> MFEARLVQGSILKKVLEALKDLINEACWDISSSGVNLQSMDSSHVSLVQLTLRSEGFDTYRCDRNLAMGVNLTSMSKILKCAGNEDIITLRAEDNADTLALVFEAPNQEKVSDYEMKLMDLDVEQLGIPEQEYSCVVKMPSGEFARICRDLSHIGDAVVISCAKDGVKFSASGELGNGNIKLSQTSNVDKEEEAVTIEMNEPVQLTFALRYLNFFTKATPLSSTVTLSMSADVPLVVEYKIADMGHLKY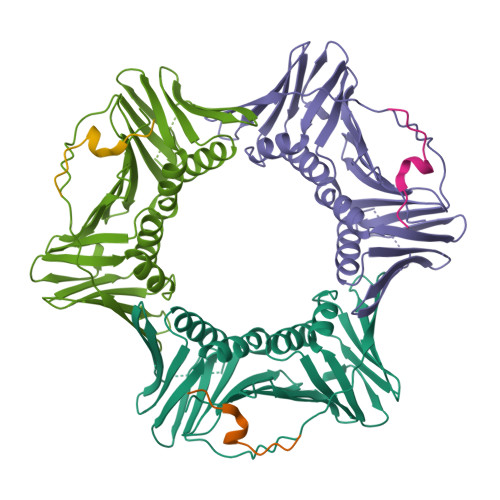YLAPKIEDEEGS;> SRQGSTQGRLDDFFKVTGSL3-OXO-PENTADECANOIC ACID | C15 H28 O3 | 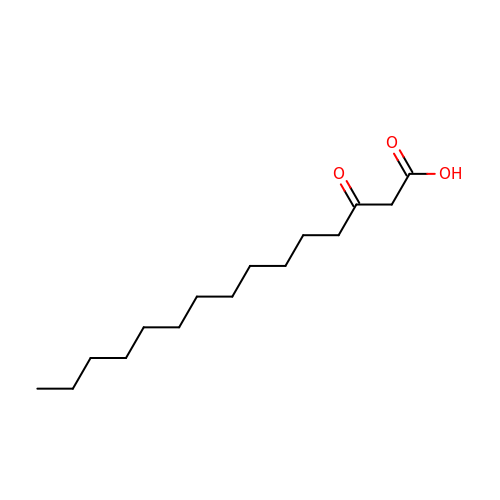CJTNJZWHYGHVCD-UHFFFAOYSA-N>[2x]MEQSIKSKGFEHRLLLIMWGLLLSLSAFAQQITVKGHVVDATGEPVIGASVIEGKSTNGTITDIDGNFSLNVSANSALTISFVGYKTQTVSVNGKTALKVTLQEDTEVLDEVVVVGYGTMKKSDLTGAVSSVGVKDIKDSPVANIGQAMQGKVSGVQIIDAGKPGDNVTIKIRGLGTINNSNPLVVIDGIPTDLGLSSLNMADVERVDVLKDASATAIYGSRGANGVVMITSKRGAEGAGKVTVNANWAIQNATKVPDMLNAAQYAALSNDMLSNNDDNTNPYWADPSSLGKGTNWLDEMLRTGVKQSYSVSYSGGTEKAHYYVSGGFLDQSGIVKSVNYRRFNFQANSDAQVNKWLKFTTNLTFSTDVKEGGTYSIGDAMKALPTQPVKNDDGSWSGPGQEAQWYGSIRNPIGTLHMMTNETKGYNFLANITGEITFTKWLKLKSTFGYDAKFWFADNFTPAYDWKPNPVEESSRYKSDNKSFTYLWDNYFVFDHTFAKKHRVGVMAGSSAQWNNYDYLNAQKNIFMFDNIHEMDNGEKMYSLGGSQSDWALLSLMARLNYSYEDKYLLTATVRRDGSSRFGKNNRWGTFPSVSLAWRVSQEDWFPKDNFLMNDLKLRVGYGVTGNQEIGNYGFVASYNTGVYPFGNNNSTALVSTTLSNPNIHWEEVRQANFGVDMSLFDSRVSLSLDAYIKNTNDMLVKASIPITSGFEDTTETFTNAGKMRNKGVEMTLRTINLKGIFSWESALTATYNKNEILDLNSETPMFINQIGNSYVTMLKAGYPINVFYGYVTDGLFQNWGEVNRHATQPGAAPGDIRFRDLNNDGVINDEDRTILGNPNPNWFFSLSNNLSYKGWELSVFLQGVAGNKIYNANNVDNEGMAAAYNQTTAVLNRWTGEGTSYSMPRAIWGDPNQNCRVSDRFVENGSYLRLKNITLSYTLPKKWLQKIQLENARISFSCENVATITRYSGFDPEVDVNGIDSSRYPISRTFSMGLNFNF

Glycan uptake across the bacterial outer membrane (OM) of these bacteria is mediated by SusCD protein complexes, comprising a membrane-embedded barrel and a lipoprotein lid, that is thought to open and close to facilitate substrate binding and transport. Here we show that for both the levan and dextran utilisation systems of Bacteroides thetaiotaomicron, the additional OM components assemble on the core SusCD transporter, forming stable glycan utilising machines which we term ‘utilisomes’. Transport-competent FOS are generated from levan by a surface-exposed lipoprotein, a GH32-family levan endo-glycanase (GHlev), while an SGBP (SGBPlev) is thought to recruit levan at the cell surface. Single particle cryogenic electron microscopy (cryoEM) structures in the absence and presence of substrate reveal concerted conformational changes that demonstrate the mechanism of substrate capture, and rationalise the role of each component in the utilisome.

Initial biochemical characterisation indicated that a utilisome existed, but cryoEM of the dextran complex revealed it to be much more aggregation prone than the levan utilisome. Despite this, initial 3D classification revealed that the SusCDdex complex is intact, (i.e. a SusC2D2 tetramer), and that the SusDdex lids are open. The positions of GHdex and SGBPdex were initially assigned by rigid-body docking of AlphaFold2-predicted models into additional density decorating the lip of SusCdex. However, unlike in the levan system, no classes corresponding to an octameric dextran utilisome existed, which we attribute to a higher propensity of the dextran utilisomes to disassemble/aggregate, potentially at the air-water interface during cryoEM grid preparation. We did observe heptameric complexes, containing two copies of the SGBPdex and a single GHdex (ED Fig. 6a-d), together with hexamers and pentamers encompassing all possible complements of GHdex and SGBPdex (ED Fig. 6e). For levan, GHlev is nearest to the hinge of SusDlev, whereas for dextran, the SGBPdex is nearest to SusDdex. Despite this variation, for two distinct Bacteroides PULs these data show that all OM components required for utilisation of a glycan are assembled into a utilisome.>[2x]SVKERTEQIEHILKSSVVKVAYGSSNPKRSEPDLNILKDLIDSNYVVFDVLLQFLTHQDPVVTAAAAQVYIRRAYRAYTIGDIRVHEGVTVPIVEWKFQLPSAAFSTFPTVKSKMGMNRAVSVSDLSYVANSQSSPLREGILMAVDHLDDVDEILSQSLEVIPRHQSSSNGPAPD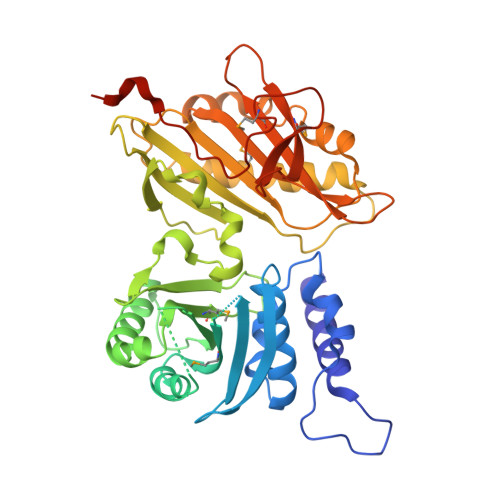RSGSSASLSNVANVCVASTEGFESEEEILVRLREILDLNKQELINASIRRITFMFGFKDGSYPKYYTFNGPNYNENETIRHIEPALAFQLELGRLSNFNIKPIFTDNRNIHVYEAVSKTSPLDKRFFTRGIIRTGHIRDDISIQEYLTSEANRLMSDILDNLEVTDTSNSDLNHIFINFIAVFDISPEDVEAAFGGFLERFGKRLLRLRVSSAEIRIIIKDPQTGAPVPLRALINNVSGYVIKTEMYTEVKNAKGEWVFKSLGKPGSMHLRPIATPYPVKEWLQPKRYKAHLMHHHHHH> GSHMASMFGKLREKLKSFVKRVEEEVEKEEEEVEKKGLLDRILTVEIKEKDVDKALDELEIDLLEADVALEVVDALREKIKQKLVGKKVRIGTDKGKIIEEAVKEAVSEILETSRRIDLIEEIRKAEKPYVIMFVGFNGSGKTTTIAKLANWLKNHGFSVVIAASDTFRAGAIEQLEEHAKRIGVKVIKHSYGADPAAVAYDAIQHAKARGIDVVLIDTAGRSETNRNLMDEMKKIARVTKPNLVIFVGDALAGNAIVEQARQFNEAVKIDGIILTKLDADARGGAALSISYVIDAPILFVGVGQGYDDLRPFEKEWFLERIFGEENA

The process is mediated by evolutionarily related signal recognition particles (SRPs) and their cognate membrane-associated receptors (SRs also called FtsYs in Bacteria and Archaea). The core proteins of SRPs and SRs are GTPases that each contain a structurally and functionally conserved NG domain where the G domain adopts a ras-like fold responsible for GTP binding and the N-domain adopts a four α-helix bundle fold. Here we describe the X-ray structures and solution conformations of FtsY, the SR from the hyper-thermophilic archaeon Pyrococcus furiosus (Pfu), in its free and GDP•magnesium-bound forms. The low resolution, solution scattering data complements our high-resolution crystallographic analysis and shows that the crystallographic structure and the average conformation adopted in solution are similar. While the overall architecture of the archeal receptor resembles its previously described bacterial homologues from the SRP/SR GTPases family, the structure of Pfu-FtsY reveals novel features: The elongated N domain lacks the N-terminal extension observed in all other bacterial FtsYs and is instead characterized by a long N-terminal helix αN1 that packs against the NG core in a different way; sequence analysis suggests that archeal receptors may cluster apart from their bacterial homologues.

We tried to co-crystallize Pfu-FtsY in presence of GTP. Although SRP-GTPases, especially the SR subgroup, are distinguished by their low intrinsic GTPase activity and nucleotide specificity, the crystal structure we obtained showed the presence of GDP•magnesium bound in the catalytic site suggesting that nucleotide hydrolysis took place during the course of crystallization. Identical crystals could be obtained in presence of GDP but not in presence of non-hydrolyzable GTP analogs. The resulting structure was solved at 2.0Å resolution by molecular replacement using the apo structure as template. The previously reported Taq-FtsY•GDP structure was obtained with a receptor that lacked the first 20 aminoacids and contained no magnesium, which is required for the association between FtsY and Ffh.. The structure reveals two nucleotide molecules, one in the catalytic site and one located at the surface of the protein next to the IBD motif unique to all SRP-GTPases. The refined occupancies of 100% (catalytic GDP) and 69% (external GDP) and atomic displacement factors of the two GDPs are indicated. The GDP•magnesium bound receptor adopts a conformation close to the one observed in the Taq-FtsY•Ffh complex. Our FtsY structure identified a second and distinct external nucleotide-binding site located on the surface of the receptor.N-[4-[(4-naphthalen-2-yloxyphenyl)sulfamoyl]phenyl]ethanamide | C24 H20 N2 O4 S | 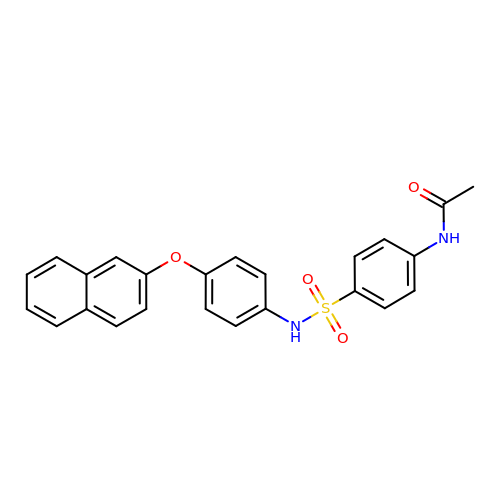YYGHDFIKAKVWFF-UHFFFAOYSA-N>MVKLMEVYEGKAKKMIPIDDDKLIMEFKDDATAFDGTKKARFKGKGWLNAQLSVIFFKLLEEHGIKTHFIGVAGGNRLIVEKLDMYPLEVVVRNVVAGSLKKRLPLPEGYELPEPIVELYYKNDELHDPMINYYHAKVLGISLDEIKKIEEIALKVNEILKDYLAKKGIILVDFKLEFGKDKNGDIVLADEISPDTCRFWDAKTKRSLDKDVFRFDKGDLIE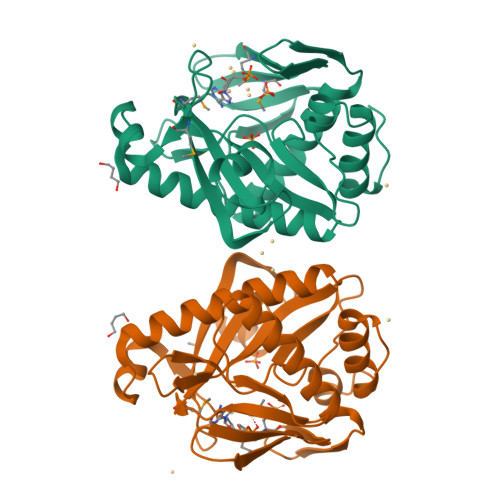AYKEIYERITGEKPEF[2x]>VEGRFQLVAPYEPQGDQPQAIAKLVDGLRRGVKHQTLLGATGTGKTFTISNVIAQVNKPTLVIAHNKTLAGQLYSELKEFFPHNAVEYFVSYYDYYQPEAYVPQTDTYIEKDAKINDEIDKLRHSATSALFERRDVIIVASVSSIYGLGSPEEYRELVVSLRVGMEIERNALLRRLVDIQYDRNDIDFRRGTFRVRGDVVEIFPASRDEHSIRVEFFGDEIERIREVDALTGEVLGEREHVAIFPASHFVCREEKMRLAIQNIEQELEERLAELRAQGKLLEAQRLEQRTRYDLEMMREMGFSSGIENYSRHLALRPPGSTPYTLL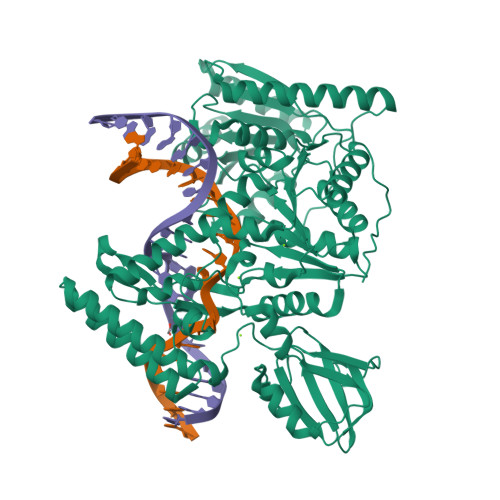DYFPDDFLIIVDESHVTLPQLRGMYNGDRARKQVLVDHGFRLPSALDNRPLTFEEFEQKINQIIYVSATPGPYELEHSPGVVEQIIRPTGLLDPTIDVRPTKGQIDDLIGEIRERVERNERTLVTTLTKKMAEDLTDYLKEAGIKVAYLHSEIKTLERIEIIRDLRLGKYDVLVGINLLREGLDIPEVSLVAILDADKEGFLRSERSLIQTIGRAARNANGHVIMYADTITKSMEIAIQETKRRRAIQEEYNRKHGIVPRTVKKEIR[2x]>MPIHNLNHVNMFLQVIASGSISSAARILRKSHTAVSSAVSNLEIDLCVELVRRDGYKVEPTEQALRLIPYMRSLLNYQQLIGDIAFNLNKGPRNLRVLLDTAIPPSFCDTVSSVLLDDFNMVS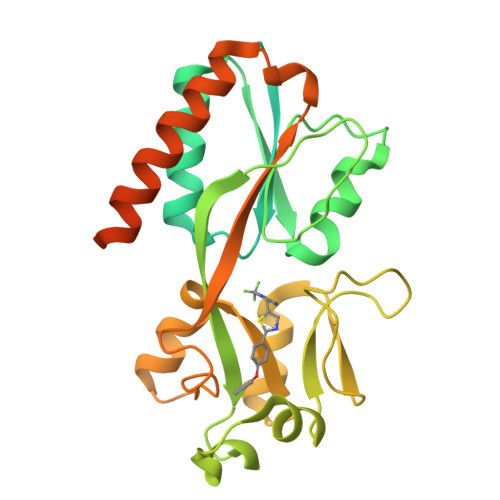LIRTSPADSLATIKQDNAEIDIAITIDEELKISRFNQCVLGYTKAFVVAHPQHPLCNASLHSIASLANYRQISLGSRSGQHSNLLRPVSDKVLFVENFDDMLRLVEAGVGWGIAPHYFVEERLRNGTLAVLSELYEPGGIDTKVYCYYNTALESERSFLRFLESARQRLRELGRQRFDDAPAWQPSIVETAQRRSGPKALAYRQRAAPE[2x]> ASMYLKEIFVDNFRNLKKQKLEFCEGVNLIYGLNAQGKSNLLEAIRLLSMGRSFRGSKMSELVKFDEEYFYVRGLVRSADFYEKKIEFGYKVNGNKVIKVNGNKLKSTGEILGHFLTVIFSPEDIEIIKEGPSRRRKYLDACISVIDKNYFFDLLQYNKTLSNRNSLLKKIKEEGKGEDLLEIFDEKLAEYGARIIKVRNNYLEKLKNSMSKFLMEISNEKLEIIYLNSAGVKEVHEENLIREKLKNRLTKSLTLDLKYLSTQVGPHREDFKILINGYDSRVYSSQGQKRTAALCLKLSELEILEEETGEKPVLLLDDVMSELDD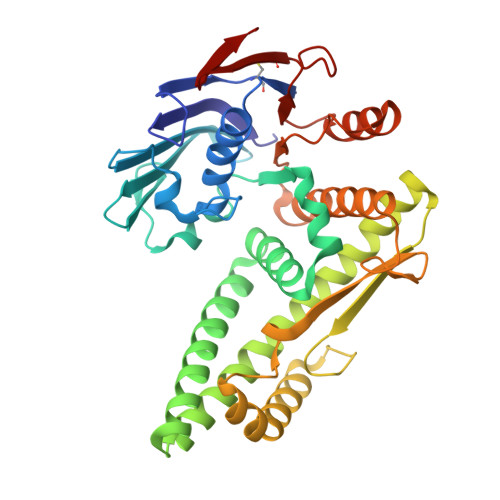NRKKYILKKLEGFQSFITHTSKSDVEGDCCFKIYDGIVDKLA> MVDWRLFEPLFNWARKKSLWIVAFCTGCGGIEMPPLMTARYDLERFGIMPDPSPRQYDLFLITGYVTPKTLKRIIITYEMAPDPKYVLAHGSCPINGGIYWDAYNAIKQLDKYIPVDVYIAGCMPRPEAVMDGIKKLMEMIENGEADGWKRYK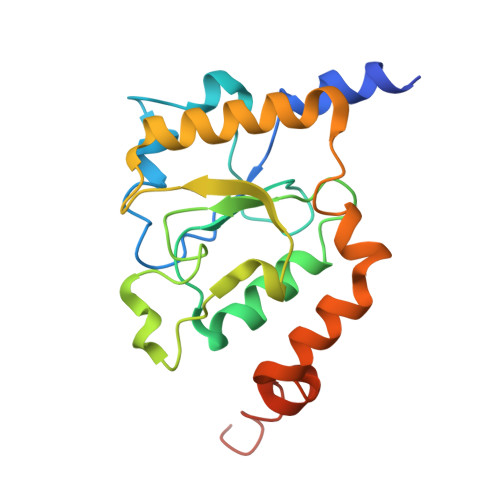ENYEWYRKNQDELLGEGWREKEARKWIPWLMDKRKEVKE>TIEKPKISVAFICLGNFCRSPMAEAIFKHEVEKANLENRFNKIDSFGTSNYHVGESPDHRTVSICKQHGVKINHKG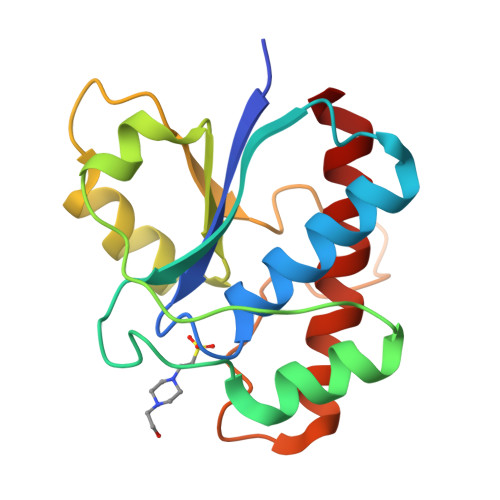KQIKTKHFDEYDYIIGMDESNINNLKKIQPEGSKAKVCLFGDWNTNDGTVQTIIEDPWYGDIQDFEYNFKQITYFSKQFLKKEL[2x]> GTGDGSMTLQITETYERLRASHISRWG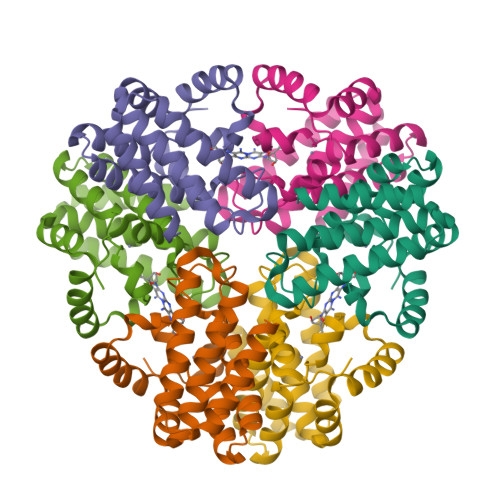IVQTTYPQNIAEHMWRVWLLCRDWGAAAGMPQHTVRQACEFALVHDLAEIRTGDAPTPHKTPELKELLAGIEAQIVPEVAELEATMAPEARELWKFCDTAEAVLFLKVNGLGAHAYDVQHLLMEQMKRRLMDSVLDVEVQDELMFQFERTIKKT> GPHMTRIIYDRKFLMECRNSPVTK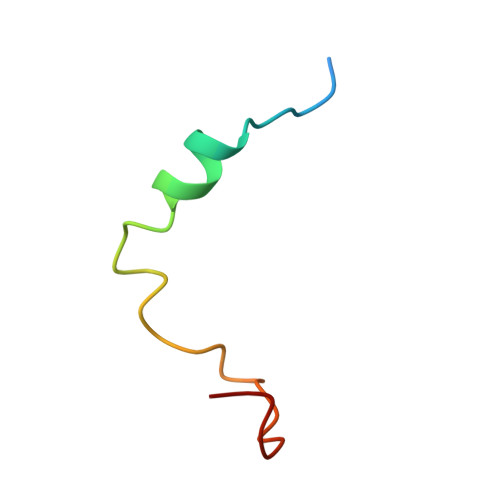TPPRDLPTIPGVTS> PETRPNHTIYINNLNEKIKKDELKKSLHAIFSRFGQILDILVSRSLKMRGQAFVIFKEVSSATNALRSMQGFPFYDKPMRIQ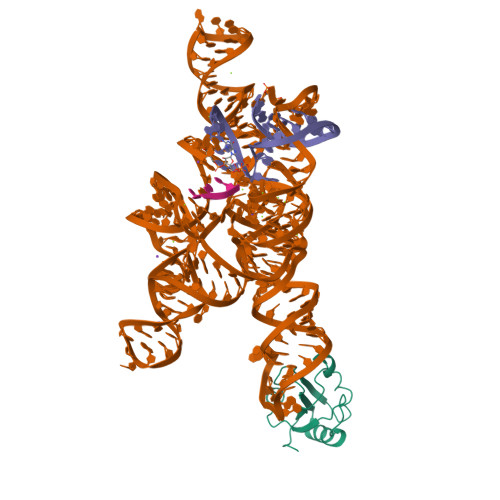YAKTDSDIIAKMK>[5x]SVTVKRIIDNTVIVPKLPANEDPVEYPADYFRKSKEIPLYINTTKSLSDLRGYVYQGLKSGNVSIIHVNSYLYGALKDIRGKLDKDWSSFGINIGKAGDTIGIFDLVSLKALDGVLPDGVSDASRTSADDKWLPLYLLGLYRVGRTQMPEYRKKLMDGLTNQCKMINEQFE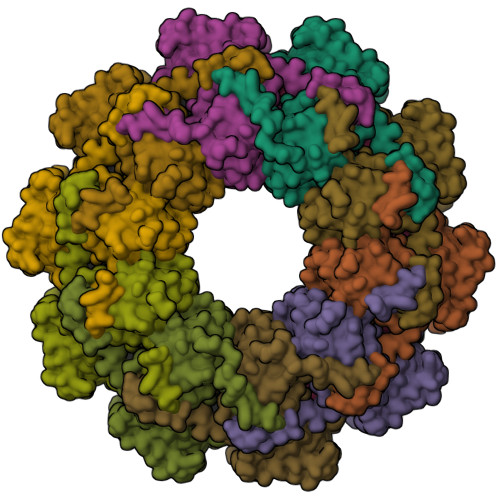PLVPEGRDIFDVWGNDSNYTKIVAAVDMFFHMFKKHECASFRYGTIVSRFKDCAALATFGHLCKITGMSTEDVTTWILNREVADEMVQMMLPGQEIDKADSYMPYLIDFGLSSKSPYSSVKNPAFHFWGQLTALLLRSTRARNARQPDDIEYTSLTTAGLLYAYAVGSSADLAQQFCVGDNKYTPDDSTGGLTTNAPPQGRDVVEWLGWFEDQNRKPTPDMMQYAKRAVMSLQGLREKTIGKYAKSEFDK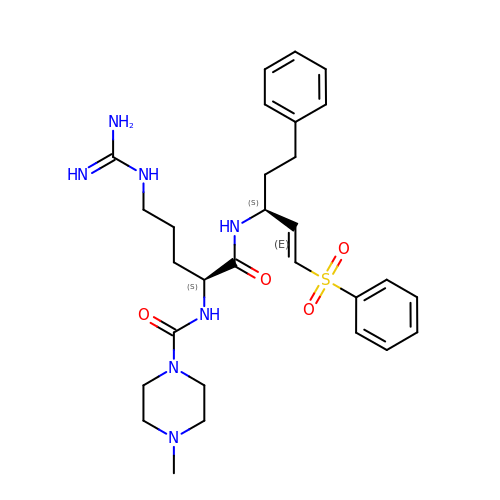(Z)-N-(5-GUANIDINO-1-OXO-1-(5-PHENYL-1-(PHENYLSULFONYL)PENT-1-EN-3-YLAMINO)PENTAN-2-YL)-4-METHYLPIPERAZINE-1-CARBOXAMIDE | C29 H41 N7 O4 S | QLVPCZICLZOVOF-GQCXWPLSSA-N> GSHMSGIALSRLAQERKAWRKDHPFGFVAVPTKNPDGTMNLMNWECAIPGKKGTPWEGGLFKLRMLFKDDYPSSPPKCKFEPPLFHPNVYPSGTVCLSILEED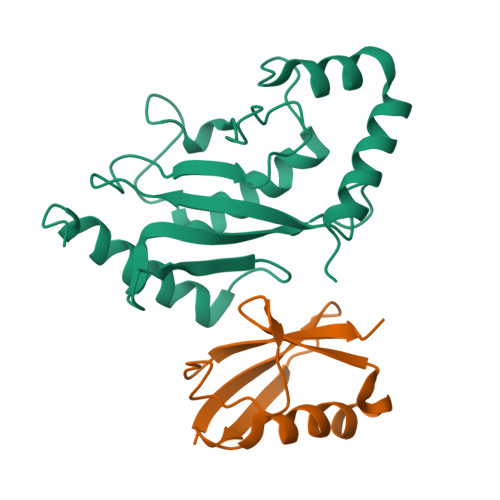KDWRPAITIKQILLGIQELLNEPNIQDPAQAEAYTIYCQNRVEYEKRVRAQAKKFAPS;> MSDQEAKPSTEDLGDKKEGEYIKLKVIGQDSSEIHFKVKMTTHLKKLKESYCQRQGVPMNSLRFLFEGQRIADNHTPKELGMEEEDVIEVYQEQTGG(E,2S)-N-methyl-5-(5-phenoxy-3-pyridyl)pent-4-en-2-amine 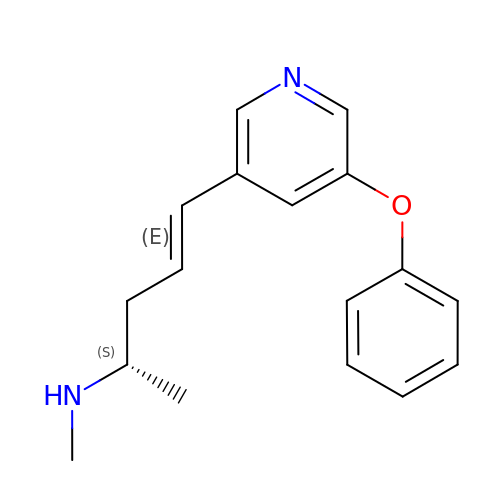| C17 H20 N2 O | MVYJEPAEKWWVOZ-OWNNVSBGSA-N7-ethoxy-7-oxidanylidene-heptanoic acid | C9 H16 O4 | 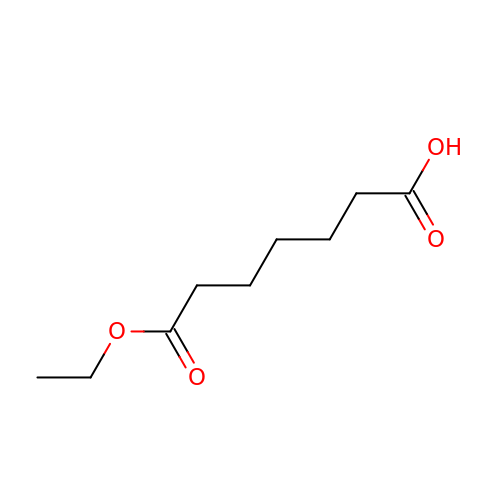NQYXFXWKKYGBNL-UHFFFAOYSA-N Delivery of these newly synthesized hydrolytic enzymes to lysosomes depends on the P-type lectins, 300-kDa cation-independent mannose 6-phosphate receptor (CI-MPR) and 46-kDa cation-dependent MPR (CD-MPR), that bind the carbohydrate determinant, mannose 6-phosphate (M6P), on lysosomal enzymes. CI-MPR’s extracytoplasmic region contains 15 homologous domains called “mannose 6-phosphate receptor homology” domains (MRH) due to their similar size (~150 residues) and conserved residues, including disulfide bonding. CI-MPR has four non-adjacent CRDs (domains 3, 5, 9, and 15), each with distinctive phosphomonoester and phosphodiester glycan preferences. We now report the crystal structures of the N-terminal five domains of human CI-MPR, revealing the orientation of two CRDs (domains 3 and 5) with respect to each other at pH 5.5 and 7.0.

Crystallization screening of human CI-MPR domains 1–5 protein in the presence of 10-mM M6P resulted in two conditions yielding diffraction quality crystals. Interestingly, both conditions show evidence of the N-glycan at N591 of a crystallographic neighbor partially occupying the carbohydrate-binding site of domain 5. The pH 5.5 structure had sufficient occupancy to allow carbohydrate refinement while the corresponding region in the pH 7.0 structure did not. The other CRD (domain 3) remains unoccupied in both structures, unlike bovine CI-MPR domains 1–3, where we showed domain 3 was bound to a ligand: either M6P or the oligosaccharide of a crystallographic neighbor (inset). Although we were surprised that the domain-3 binding pocket did not contain M6P at pH 7.0 conditions, the presence of the N-linked glycan near the binding site of domain 5 could perturb conformational equilibria between substructures that stabilize a domain arrangement most favorable for crystallographic packing. The interdomain linker between domains 2 and 3 adopts a more extended structure in the absence of ligand, allowing for the repositioning of domain 3. In the absence of a ligand bound to domain 3, its C-terminal face contacts the C-terminal face of domain 1. The flexibility of domain 4 was also recently demonstrated in the cryo-EM structures published by Wang et al. at the time of this paper’s submission. Comparing their bovine domains 4–14 structure at pH 7.4 in the presence of IGF2 with our human domains 1–5 structure at pH 5.5 or 7.0 shows domain 4 rotated ~180°. Another possibility is that PPT1 binding to domain 3 causes a rearrangement of domains such that the binding site of domain 5 is no longer accessible by ligand. This latter possibility of allosteric interactions between the CRDs is consistent with our crystal structures that illustrate that domain interactions can be dramatically altered in the presence or absence of ligands, such as between domain 3 and domains 1 and 2.

> AAGSTQAQAAPFPELCSYTWEAVDTKNNVLYKINICGSVDIVQCGPSSAVCMHDLKTRTYHSVGDSVLRSATRSLLEFNTTVSCDQQGTNHRVQSSIAFLCGKTLGTPEFVTATECVHYFEWRTTAACKKDIFKANKEVPCYVFDEELRKHDLNPLIKLSGAYLVDDSDPDTSLFINVCRDIDTLRDPGSQLRACPPGTAACLVRGHQAFDVGQPRDGLKLVRKDRLVLSYVREEAGKLDFCDGHSPAVTITFVCPSERREGTIPKLTAKSNCRYEIEWITEYACHRDYLESKTCSLSGEQQDVSIDLTPLAQSGGSSYISDGKEYLFYLNVCGETEIQFCNKKQAAVCQVKKSDTSQVKAAGRYHNQTLRYSDGDLTLIYFGGDECSSGFQRMSVINFECNKTAGNDGKGTPVFTGEVDCTYFFTWDTEYACVKEKEDLLCGATDGKKRYDLSALVRHAEPEQNWEAVDGSQTETEKKHFFINICHRVLQEGKARGCPEDAAVCAVDKNGSKNLGKFISSPMKEKGNIQLSYSDGDDCGHGKKIKTNITLVCKPGDLESAPVLRTSGEGGCFYEFEWHTAAACVLSKTEGENCTVFDSQAGFSFDLSPLTKKNGAYKVETKKYDFYINVCGPVSVSPCQPDSGACQVAKSDEKTWNLGLSNAKLSYYDGMIQLNYRGGTPYNNERHTPRATLITFLCDRDAGVGFPEYQEEDNSTYNFRWYTSYACPEEALVPL> GPTVVDQIRLWQ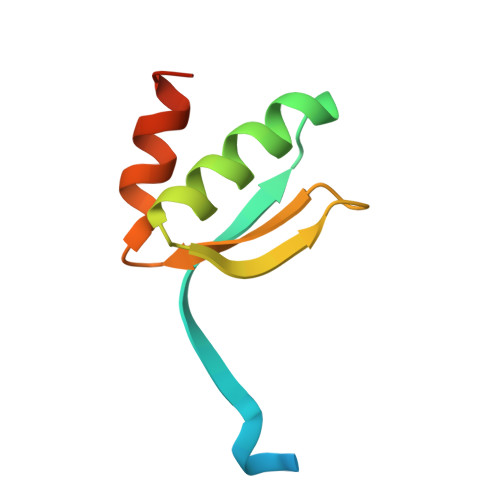LELDRVITYEGSLYSDFETSQEYNLLSKYAQDIGVLLWKDDKKKKFFISKEGNSQVLDFAKRKLKKKQ>MAHPGRTGYD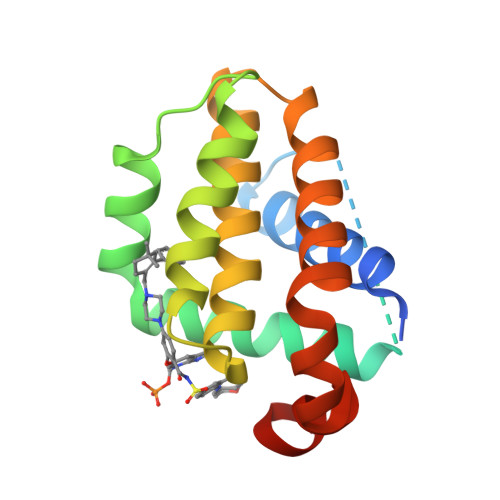NREIVMKYIHYKLSQKGYEWDAGDDVEENRTEAPEGTESEVVHLTLRQAGDDFSRRYRRDFAEMSSQLHLTPFTARGRFATVVEELFRDGVNWGRIVAFFEFGGVMCVESVNREMSPLVDNIALWMTEYLNRHLHTWIQDNGGWDAFVELYGPSMR[3x]> SNAEDDKLKSVEALRQKGNELFVQKDYKEAIDAYRDALTRLDTLILREKPGEPEWVELDRKN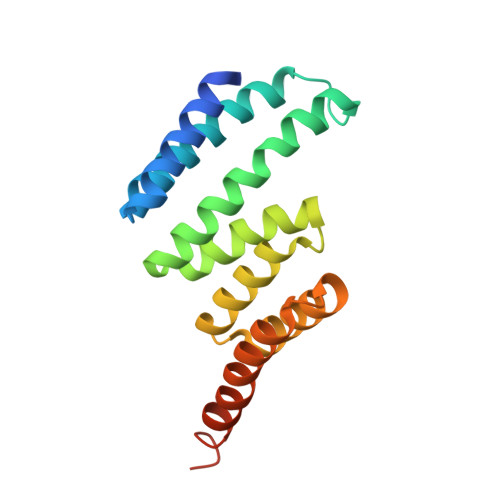IPLYANMSQCYLNIGDLHEAEETSSEVLKREETNEKALFRRAKARIAAWKLDEAEEDLKLLLRNHPAAASVVAREMKIVTERRAEKKADSRVTYSKMFQP>[3x]AQVINTFDGVADYLQTYHKLPDNYITKSEAQALGWVASKGNLADVAPGKSI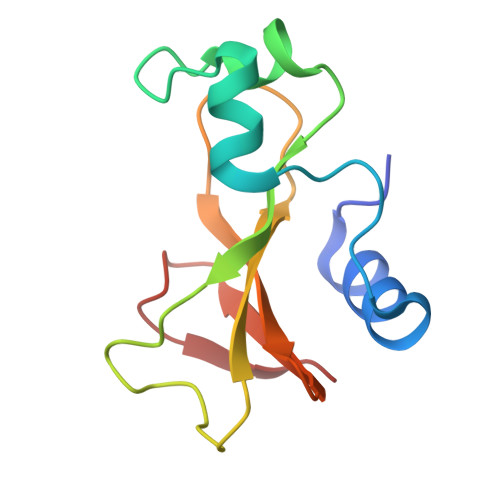GGDIFSNREGKLPGKSGRTWREADINFTSGFRNSDRILYSSDWLIYKTTDHYQTFTKIR>GPHMGGSAEVNASPLKHFVTAKKKINGIFEQLGAYIQESATFLEDTYRNAELDPVTTEEQVLDVKGYLSKVRGISEVLARRHMKVAFFGRTSNGKSTVINAMLWDKVLPSGIGHTTNCFLRVEGTDGHEAFLLTEGSEEKRSAKTVNQLAHALHQDKQLHAGSLVSVMWP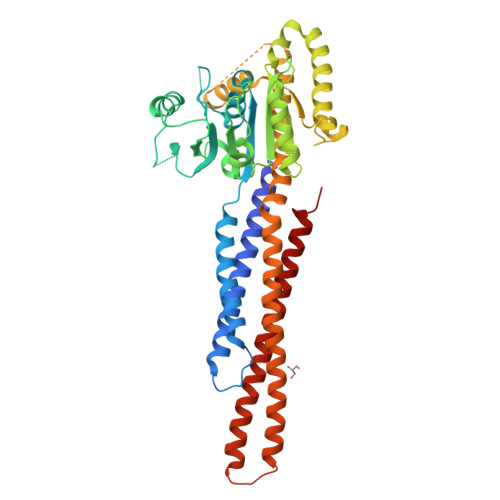NSKCPLLKDDLVLMDSPGIDVTTELDSWIDKFCLDADVFVLVANSESTLMQTEKHFFHKVSERLSRPNIFILNNRWDASASEPEYMEEVRRQHMERCTSFLVDELGVVDRSQAGDRIFFVSAKEVLNARIQKAQGMPEGGGALAEGFQVRMFEFQNFERRFEECISQSAVKTKFEQHTVRAKQIAEAVRLIMDSLHMAAREQQVYCEEMREERQDRTRENLEQEIAAMNKKIEVLDSLQSKAKLLRNKAGWLDSELNMFTHQYLQPSR[4x]During previous studies, we identified and characterized a highly reactive self-splicing group IA1 intron that is found within the mitochondrial rRNA of Candida albicans (C.a.mtLSU), representing a potential pan-fungal drug target due to its wide presence in diverse species of ascomycetes pathogenic fungi. To elucidate the mechanism of action, intron splicing rate was monitored as a function of compound 1 and guanosine cofactor, which is the nucleophile required for activity of all group I introns. The cryoEM reconstruction revealed a canonical 3D arrangement for group I intron structures with three main coaxially stacked RNA helices that encompass the intron core. However, in this case, we also visualized two distinctive structural modules (P7ext and P9.1) that brace the intron active site, which provide extensive mechanical support to the intron core and potentially explain the unusually robust biochemical activity of the C.a.mtLSU intron.

Before embarking on structural studies of the hit series, it was important to first establish the molecular interaction network between the C.a.mtLSU intron and guanosine itself using cryoEM. Here, we used calcium as the metal ion to trap the unspliced precursor RNA (the intron flanked by intact exons) bound to guanosine monophosphate (GMP). From this dataset, we obtained a 3.1Å reconstruction and built the atomic model of the intron RNA containing the bound guanosine ligand. In the structural model, the 3′-OH on bound guanosine, which serves as the reaction nucleophile, is close to the scissile phosphate with the corresponding catalytic metal MC in place, indicating that the visualized structure is near the precatalytic state prior to the first step of splicing. One of these interactions is the P11 pseudoknot, which anchors the P7ext helix against the extended P6 stem, effectively stapling the structural and catalytic domains of the intron together. Supporting this pseudoknot is a tertiary interaction between P9.1 and P7ext mediated by A-minor motifs in which a network of 2′-OHs form long-range interactions with the nucleobase of A293. Finally, a unique stacking sandwich featuring noncanonical base pairs from four different RNA strands (P3, P7, P7ext, and J8/7) interdigitates the catalytic helices. In contrast, guanosine has a weaker interaction network, engaging the phosphate of A152 through a single hydrogen bond with its 2′-OH. Through comparison of the two liganded structures of the intron RNA, we showed that the overall structural fold of the intron is preserved while the largest conformational change involves the P1 helix, which consists of the 5′-exon and the intronic internal guide sequence (IGS).

> CGCUAGGGAUAAACUGUUUGUCCCUUUAUAUAGAGAUAUAUAGAAUAACAAUCGGGUGAAUUGCAAGAAUACCACCCACCUCCUUUGGAGGUGGGUGACAAUUUGCAGCGAAGUAUAUAUUAGCUUAAUAAUAAAAUAUUAUUUAGAUAUAUAAACGUUCAACGACUAGAAGGUGAGUAAGCUAACAAUAACCCUUCCACGAGCGCCCGACAUCUUAAUGAACCAACAAUUACAAUUAAUUAAAGGUCAUUAUGAUGAUGACAUAGUCUGAACUAAAUAGUGAUAUUUAGAUAUAAUAUUUAAAUGAUAUUAUGAUAACAAAAUUGAACAGG>[2x]MSKAVPAIILVRPQLGENIGKAARAMLNFGLDDLRLVAPRDGWPNPSAGPAASGADRVLQQARVFPTVAEAVADCAHVYATTVRKRGVTKPVMT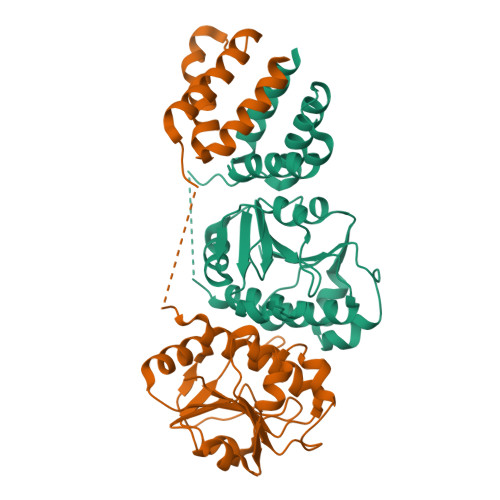PEQAAQTIHEQEGGVGILFGPERAGLETDDVALARTIITVPVNPEFSSLNLAQAVILVAYEWSKGQTLAQPTKVDMEPPAPQEELEAMIGHLENMLDKNGYFFPIPRIPTIKRTLRTLLTKPSWNSMEIRTLRGVLSTLEKPRHNAHKG>[2x]MELIKGQALFLELD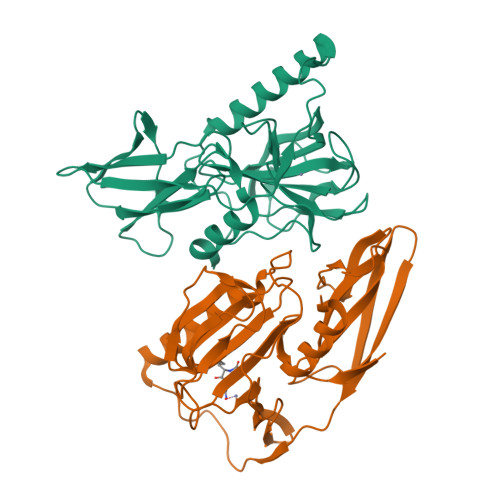KKDFLSLKNNDKNIPTFAHPKNQEKILAIFSLPYKNPPQNTKLIAFYKDKKEEIFIKTLEGNYKSEKLQVENKKIFPPKTIQERIAKELKEANAIYSSYTPKALFNGAFNIPLNSFITSDFGKARTFNEKVASYHSGTDFRAATGTPIYAANSGVVKIAKDRYFAGNSVVIDHGFGIYSQYYHLSKIDVKVGQKIKKGELIGLSGASGRVSGPALHFGILAGGKQVDPLDFVSKFNAIFQL> MLIGSHVSPTDPLAAAEAEGADVVQIFLGNPQSWKAPKPRDDAAALKAATLPIYVHAPYLINLASANNRVRIPS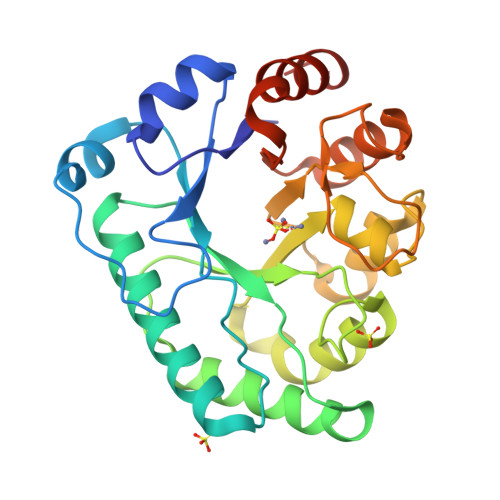RKILQETCAAAADIGAAAVIVHGGHVADDNDIDKGFQRWRKALDRLETEVPVYLENTAGGDHAMARRFDTIARLWDVIGDTGIGFCLDTCHTWAAGEALTDAVDRIKAITGRIDLVHCNDSRDEAGSGRDRHANLGSGQIDPDLLVAAVKAAGAPVICETADQGRKDDIAFLRERTGSHHHHHH> ISEFGSSRAGDKPVIGDMPA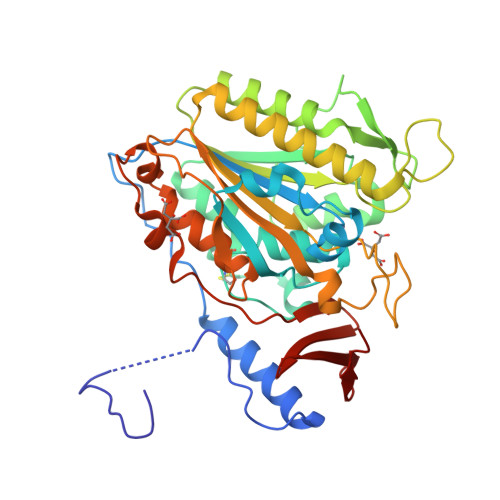QTAPPTTANLNAWLNTFYAAEEKRKTTFPAQLPPDAQPFDLLVINICSLSWSDVEAAGLMSHPLWSHFDILFKHFNSGTSYSGPAAIRLLRASCGQPSHTRLYQPANNECYLFDNLAKLGFTQHLMMDHNGEFGGFLKEVRENGGMQSELMNQSGLPTALLSFDGSPVYDDLAVLNRWLTGEEREANSRSATFFNLLPLHDGNHFPGVSKTADYKIRAQKLFDELDAFFTELEKSGRKVMVVVVPEHGGALKGDRMQISGLRDIPSPSITNVPAGVKFFGMKAPHEGAPIDINQPSSYLAISELVVRAVDGKLFTEDSVNWNKLTSNLPQTAPVSENANAVVIQYQGKPYVRLNGGDWVPYPQ> MESSTYQERADELVVKIKDMFNALGDGDISPSAYDTAWVARLATISSDGSEKPRFPQALNWVFNNQLQDGSWGIESHFSLCDRLLNTTNSVIALSVWKTGHSQVQQGAEFIAENLRLLNEEDELSPDFQIIFPALLQKAKALGINLPYDLPFIKYLSTTREARLTDVSAAADNIPANMLNALEGLEEVIDWNKIMRFQSKDGSFLSSPASTACVLMNTGDEKCFTFLNNLLDKFGGCVPCMYSIDLLERLSLVDNIEHLGIGRHFKQEIKGALDYVYRHWSERGIGWGRDSLVPDLNTTALGLRTLRMHGYNVSSDVL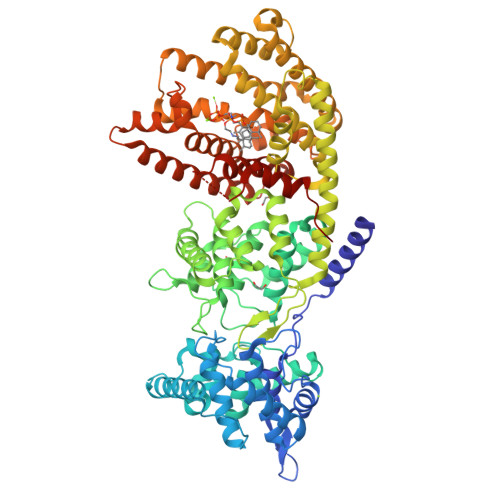NNFKDENGRFFSSAGQTHVELRSVVNLFRASDLAFPDERAMDDARKFAEPYLREALATKISTNTKLFKEIEYVVEYPWHMSIPRLEARSYIDSYDDNYVWQRKTLYRMPSLSNSKCLELAKLDFNIVQSLHQEELKLLTRWWKESGMADINFTRHRVAEVYFSSATFEPEYSATRIAFTKIGCLQVLFDDMADIFATLDELKSFTEGVKRWDTSLLHEIPECMQTCFKVWFKLMEEVNNDVVKVQGRDMLAHIRKPWELYFNCYVQEREWLEAGYIPTFEEYLKTYAISVGLGPCTLQPILLMGELVKDDVVEKVHYPSNMFELVSLSWRLTNDTKTYQAEKARGQQASGIACYMKDNPGATEEDAIKHICRVVDRALKEASFEYFKPSNDIPMGCKSFIFNLRLCVQIFYKFIDGYGIANEEIKDYIRKVYIDPIQVGSHHHHHH> STPGIVIPPQEQITQHGSPYGRCANKT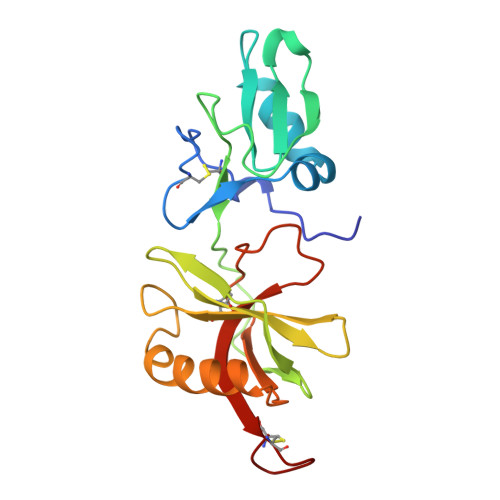RALTVAELRGSGDLQEYLRHVTRGWSIFALYDGTYLGGEYGGVIKDGTPGGAFDLKTTFCIMTTRNTGQPATDHYYSNVTATRLLSSTNSRLCAVFVRSGQPVIGACTSPYDGKYWSMYSRLRKMLYLIYVAGISVRVHVSKEEQYYDYEDATFETYALTGISICNPGSSLC> MTTKKFDEADKSNVEMYLIQAGVKQDAAATMGIWTAQELHRIKSQSYEEDYPVGSALRVFPVTTELSPTDKTFEYMTFDKVGTAQIIADYTDDLPLVDALGTSEFGKVFRLGNAYLISIDEIKAGQATGRPLSTRKASACQLAHDQLVNRLVFKGSAPHKIVSVFNHPNITKITSGKWIDASTMKPETA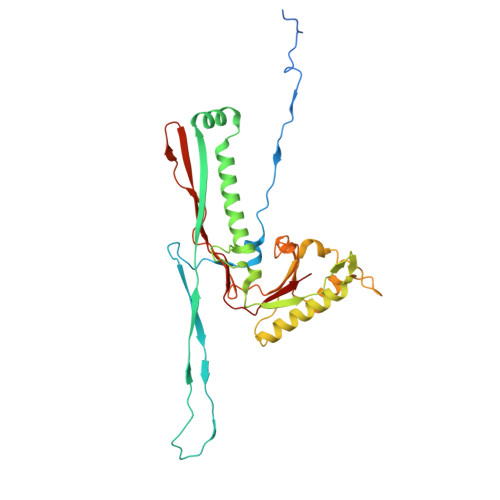EAELTQAIETIETITRGQHRATNILIPPSMRKVLAIRMPETTMSYLDYFKSQNSGIEIDSIAELEDIDGAGTKGVLVYEKNPMNMSIEIPEAFNMLPAQPKDLHFKVPCTSKCTGLTIYRPMTIVLITGV(2S)-4-[(3aR,7aS)-1,3,3a,4,5,6,7,7a-octahydroisoindol-2-yl]-4-oxidanylidene-2-(phenylmethyl)butanoic 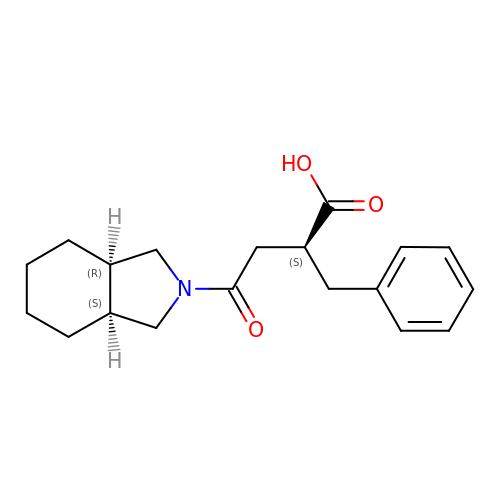acid | C19 H25 N O3 | WPGGHFDDFPHPOB-BBWFWOEESA-N>SNAERKRREKRLEETSSRLEALFENSPDMIDVLDADGTICEVNQRFCAELGYDESEVLGRSIW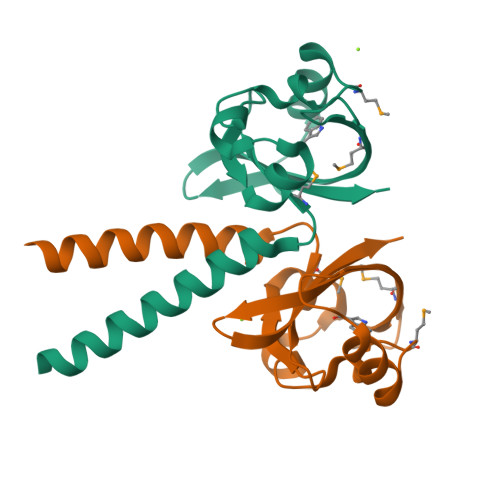EFDLMFDAEDVQTQLSGFSVDERRKFEGLYERRDGSTMSVEVHLLRFNLEGEDRFLAISRDIT[4x]Propionyl-CoA carboxylase (PCC) and 3-methylcrotonyl-CoA carboxylase (MCC) are biotin-dependent carboxylases (BDCs) that catalyze the metabolism of odd-chain fatty acids, cholesterol, and specific amino acids. In contrast, PCC and MCC have their BC, CT, and BCCP domains divided into two chains: the α subunits contain the BC and BCCP domains, with an intermediate BC-CT interaction (BT) domain between them, while the β subunits solely consist of the CT domain. In humans, PCC and MCC catalyze the carboxylation of propionyl-CoA and 3-methylcrotonyl-CoA (MC-CoA), respectively. (**A, B**) The side view (left) and top view (right) of human PCC holoenzyme (PCC-apo) (**A**) and MCC holoenzyme (MCC-apo) (**B**). Both holoenzymes are dodecamers consisting of six α subunits and six β subunits.

The cryo-EM structures of the PCC and MCC holoenzymes alone, referred to as PCC-apo and MCC-apo, were determined at resolutions of 3.02 Å and 2.29 Å, respectively ([Fig figs2], [Fig figs3], A to D and [Fig figs4], A to D, [Table tbls1] and [Table tbls2]). In human PCC holoenzyme, each α subunit binds to one β subunit containing the CT domain that can be divided into CT-N and CT-C subdomains ([Fig fig2]). The BC domain in the α subunit is situated on the CT-C subdomain, while the BCCP domain also attaches to the CT-C subdomain and positions the covalently linked biotin to a pocket adjacent to the propionyl-CoA binding pocket. The BT domain tightly interacts with both the CT-N and CT-C subdomains and functions as a hub to hold the BC and BCCP domains together with the CT domain ([Fig fig2]). A major difference between the PCC and MCC holoenzymes is that the three α subunits in each layer have no contact in the PCC holoenzyme but interact with each other in the MCC holoenzyme ([Fig fig1], A and B). Each α subunit in human PCC holoenzyme has a minor rotation relative to the corresponding α subunit in the bacteria PCC holoenzyme ([Fig fig1]). For human PCC holoenzyme, the structure in the acetyl-CoA-bound state closely resembles the structures in the apo and the propionyl-CoA-bound state. In these structures, the covalently linked biotin binds to a site (exo-site) that is distant from the catalytic residues in the CT domain, rendering it catalytically incompetent. However, we did not observe the relocation of biotin to an endo-site upon acyl-CoA binding in human PCC holoenzyme ([Fig fig3]).

>[6x]MAGFWVGTAPLVAAGRRGRWPPQQLMLSAALRTLKHVLYYSRQCLMVSRNLGSVGYDPNEKTFDKILVANRGEIACRVIRTCKKMGIKTVAIHSDVDASSVHVKMADEAVCVGPAPTSKSYLNMDAIMEAIKKTRAQAVHPGYGFLSENKEFARCLAAEDVVFIGPDTHAIQAMGDKIESKLLAKKAEVNTIPGFDGVVKDAEEAVRIAREIGYPVMIKASAGGGGKGMRIAWDDEETRDGFRLSSQEAASSFGDDRLLIEKFIDNPRHIEIQVLGDKHGNALWLNERECSIQRRNQKVVEEAPSIFLDAETRRAMGEQAVALARAVKYSSAGTVEFLVDSKKNFYFLEMNTRLQVEHPVTECITGLDLVQEMIRVAKGYPLRHKQADIRINGWAVECRVYAEDPYKSFGLPSIGRLSQYQEPLHLPGVRVDSGIQPGSDISIYYDPMISKLITYGSDRTEALKRMADALDNYVIRGVTHNIALLREVIINSRFVKGDISTKFLSDVYPDGFKGHMLTKSEKNQLLAIASSLFVAFQLRAQHFQENSRMPVIKPDIANWELSVKLHDKVHTVVASNNGSVFSVEVDGSKLNVTSTWNLASPLLSVSVDGTQRTVQCLSREAGGNMSIQFLGTVYKVNILTRLAAELNKFMLEKVTEDTSSVLRSPMPGVVVAVSVKPGDAVAEGQEICVIEAMKMQNSMTAGKTGTVKSVHCQAGDTVGEGDLLVELE;>MAAALRVAAVGARLSVLASGLRAAVRSLCSQATSVNERIENKRRTALLGGGQRRIDAQHKRGKLTARERISLLLDPGSFVESDMFVEHRCADFGMAADKNKFPGDSVVTGRGRINGRLVYVFSQDFTVFGGSLSGAHAQKICKIMDQAITVGAPVIGLNDSGGARIQEGVESLAGYADIFLRNVTASGVIPQISLIMGPCAGGAVYSPALTDFTFMVKDTSYLFITGPDVVKSVTNEDVTQEELGGAKTHTTMSGVAHRAFENDVDALCNLRDFFNYLPLSSQDPAPVRECHDPSDRLVPELDTIVPLESTKAYNMVDIIHSVVDEREFFEIMPNYAKNIIVGFARMNGRTVGIVGNQPKVASGCLDINSSVKGARFVRFCDAFNIPLITFVDVPGFLPGTAQEYGGIIRHGAKLLYAFAEATVPKVTVITRKAYGGAYDVMSSKHLCGDTNYAWPTAEIAVMGAKGAVEIIFKGHENVEAAQAEYIEKFANPFPAAVRGFVDDIIQPSSTRARICCDLDVLASKKVQRPWRKHANIPL[6x]> GSHMASMSKDEVKREAKDTDGNPEIKGERRRLHSEIQSGSLANNIKKSTVIVKDPTHIA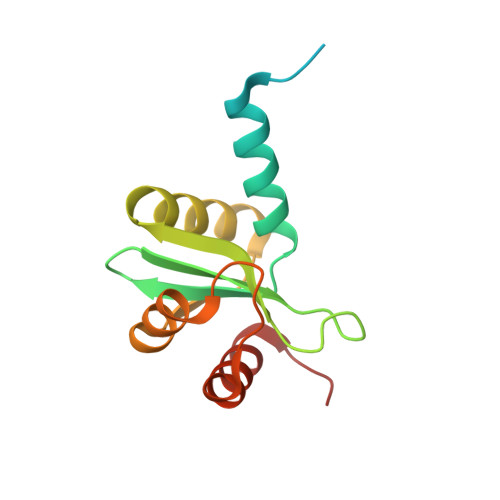ICLYYKLGETPLPLVIETGKDAKALQIIKLAELYDIPVIEDIPLARSLYKNIHKGQYITEDFFEPVAQLIRIAIDLDY>[4x]MKAVQYTEIGSEPVVVDIPTPTPGPGEILLKVTAAGLCYSDISVMDMPAAQYAYGLPLTLGHEGVGTVAELGEGVTGFGVGDAVAVYGPWGCGACHACARGRENYCTRAADLGITPPGLGSPGSMAEYMIVDSARHLVPIGDLDPVAAAPLTDAGLTPYHAISRVLPLLGPGSTAV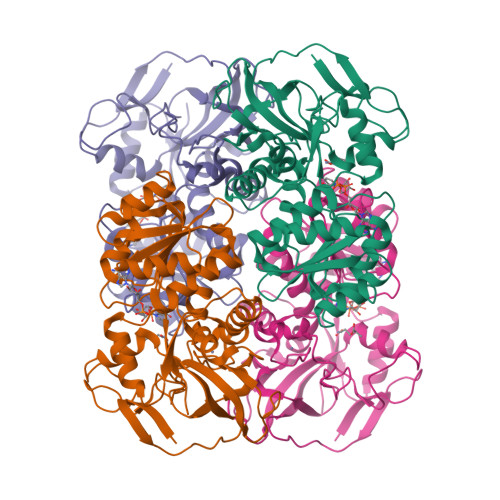VIGVGGLGHVGIQILRAVSAARVIAVDLDDDRLALAREVGADAAVKSGAGAADAIRELTGGQGATAVFDFVGAQSTIDTAQQVVAVDGHISVVGIHAGAHAKVGFFMIPFGASVVTPFAGTRSELMEVVALARAGRLDIHTETFTLDEGPAAYRRLREGSIRGRGVVVPTSHHHHH>[4x]MREKGRRQAVRGPAFMFNDRGTSLTAEEERFLDAAEYGNIPVVRKMLEESKTLNVNCVDYMGQNALQLAVGNEHLEVTELLLKKENLARIGDALLLAISKGYVRIVEAILNHPGFAASKRLTLSPCEQELQDDDFYAYDEDGTRFSPDITPIILAAHCQKYEVVHMLLMKGARIERPHDYFCKCGDCMEKQRHDSFSHSRSRINAYKGLASPAYLSLSSEDPVLTALELSNELAKLANIEKEFKNDYRKLSMQCKDFVVGVLDLCRDSEEVEAILNGDLESAEPLEVHRHKASLSRVKLAIKYEVKKFVAHPNCQQQLLTIWYENLSGLREQTIAIKCLVVLVVA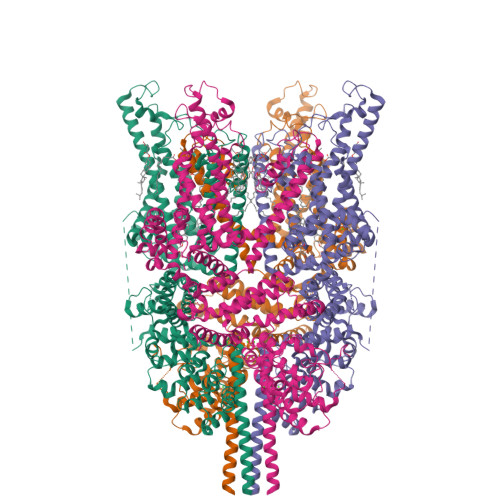LGLPFLAIGYWIAPCSRLGKILRSPFMKFVAHAASFIIFLGLLVFNASDRFEGITTLPNITVTDYPKQIFRVKTTQFTWTEMLIMVWVLGMMWSECKELWLEGPREYILQLWNVLDFGMLSIFIAAFTARFLAFLQATKAQQYVDSYVQESDLSEVTLPPEIQYFTYARDKWLPSDPQIISEGLYAIAVVLSFSRIAYILPANESFGPLQISLGRTVKDIFKFMVLFIMVFFAFMIGMFILYSYYLGAKVNAAFTTVEESFKTLFWSIFGLSEVTSVVLKYDHKFIENIGYVLYGIYNVTMVVVLLNMLIAMINSSYQEIEDDSDVEWKFARSKLWLSYFDDGKTLPPPFSLVPSPKSFVYFIMRIVNFPKCRRRRLQKDIEMGMGNSKSRLNLFTQSNSRVFESHSFNSILNQPTRYQQIMKRLIKRYVLKAQVDKENDEVNEGELKEIKQDISSLRYELLEDKSQATEELAILIHKLSEKLNPSMLRCE9H-fluorene-2,7-disulfonate | C13 H10 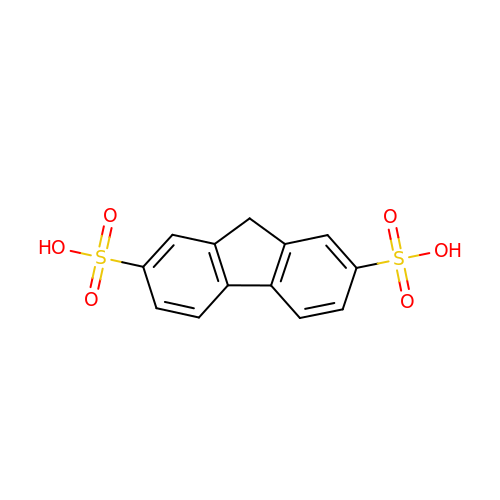O6 S2 | WBJRJWHBYUAEQD-UHFFFAOYSA-N> FMVSLPRMVYPQPKVLTPCRKDVLVVTPWLAPIVWEGTFNIDILNEQFRLQNTTIGLTVFAIKKYVAFLKLFLETAEKHFMVGHRVHYYVFTDQ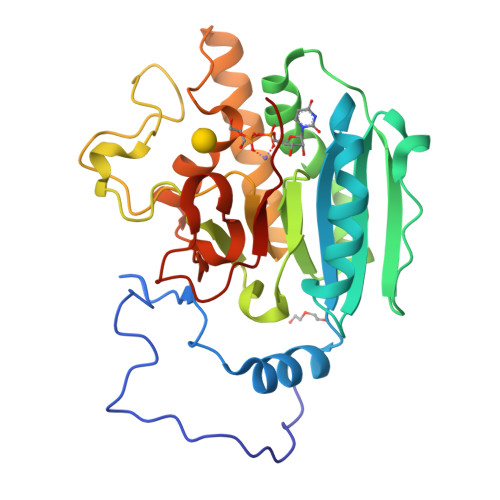PAAVPRVTLGTGRQLSVLEVRAYKRWQDVSMRRMEMISDFCERRFLSEVDYLVCVDVDMEFRDHVGVEILTPLFGTLHPSFYGSSREAFTYERRPQSQAYIPKDEGDFYYMGGFFGGSVQEVQRLTRACHQAMMVDQANGIEAVWHDESHLNKYLLRHKPTKVLSPEYLWDQQLLGWPAVLRKLRFTAVPKNHQAVRNP>[2x]MAANMYRVGDYVYFENSSSNPYLIRRIEELNKTANGNVEAKVVCFYRRRDISSTLIALADKHATLSVCYKAGPGADNGEEGEIEEEMENPEMVDLPEKLKHQLRHRELFLSRQLESLPATHIRGKCSVTLLNETESLKSYLEREDFFFYSLVYDPQQKTLLADKGEIRVGNRYQADITDLLKEGEEDGRDQSRLETQVWEAHNPLTDKQIDQFLVVARSVGTFARALDCSSSVRQPSLHMSAAAASRDITLFHAMDTLHKNIYDISKAISALVPQGGPVLCRDEMEEWSASEANLFEEALEKYGKDFTDIQQDFLPWKSLTSIIEYYYMWKTTDRYVQQKRLKAAEAESKLKQVYIPNYNKPNPNQISVNNVKAGVVNGTGAPGQSPGAGRACESCYTTQSYQWYSWGPPNMQCRLCASCWTYWKKYGGLKMPTRLDGERPGPNRSNMSPHGLPARSSGSPKFAMKTRQAFYLHTTKLTRIARRLCREILRPWHAARHPYLPINSAAIKAECTARLPEASQSPLVLKQAVRKPLEAVLRYLETHPRPPKPDPVKSVSSVLSSLTPAKVAPVINNGSPTILGKRSYEQHNGVDGNMKKRLLMPSRGLANHGQARHMGPSRNLLLNGKSYPTKVRLIRGGSLPPVKRRRMNWIDAPDDVFYMATEETRKIRKLLSSSETKRAARRPYKPIALRQSQALPPRPPPPAPVNDEPIVIED;>[2x]MAQTQGTRRKVCYYYDGDVGNYYYGQGHPMKPHRIRMTHNLLLNYGLYRKMEIYRPHKANAEEMTKYHSDDYIKFLRSIRPDNMSEYSKQMQRFNVGEDCPVFDGLFEFCQLSTGGSVASAVKLNKQQTDIAVNWAGGLHHAKKSEASGFCYVNDIVLAILELLKYHQRVLYIDIDIHHGDGVEEAFYTTDRVMTVSFHKYGEYFPGTGDLRDIGAGKGKYYAV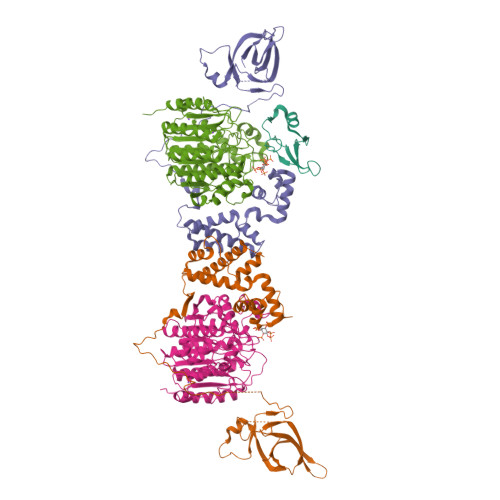NYPLRDGIDDESYEAIFKPVMSKVMEMFQPSAVVLQCGSDSLSGDRLGCFNLTIKGHAKCVEFVKSFNLPMLMLGGGGYTIRNVARCWTYETAVALDTEIPNELPYNDYFEYFGPDFKLHISPSNMTNQNTNEYLEKIKQRLFENLRMLPHAPGVQMQAIPEDAIPEESGDEDEDDPDKRISICSSDKRIACEEEFSDSEEEGEGGRKNSSNFKKAKRVKTEDEKEKDPEEKKEVTEEEKTKEEKPEAKGVKEEVKLA;> MRAHPGGGRCCPEQEEGESAAGGSGAGGDSAIEQGGQGSALAPSPVSGVRREGARGGGRGRGRWKQAGRGGGVCGRGRGRGRGRGRGRGRGRGRGRPPSGGSGLGGDGGGCGGGGSGGGGAPRREPVPFPSGSAGPGPRGPRATESGKRMDCPALPPGWKKEEVIRKSGLSAGKSDVYYFSPSGKKFRSKPQLARYLGNTVDLSSFDFRTGKMMPSKLQKNKQRLRNDPLNQNKGKPDLNTTLPIRQTASIFKQPVTKVTNHPSNKVKSDPQRMNEQPRQLFWEKRLQGLSASDVTEQIIKTMELPKGLQGVGPGSNDETLLSAVASALHTSSAPITGQVSAAVEKNPAVWLNTSQPLCKAFIVTDEDIRKQEERVQQVRKKLEEALMADILSRAADTEEMDIEMDSGDEA> AEETCFDKYTGNTYRVGDTYERPKDSMIWDCTCIGAGRGRISCTIANRCHEG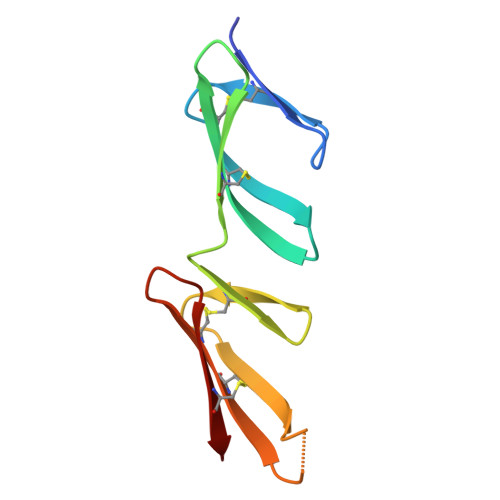GQSYKIGDTWRRPHETGGYMLECVCLGNGKGEWTCKPI>[3x]GLPRVAVDLVAPPLVHPHSQVAAGAPKVVQFRMSIEEKKMVADDDGTTAQAMTFNGSVPGPTLVVHEGDYIELTLVNPATNSMPHNVDFHAATGALGGAGLTQVVPGQEAVLRFKADRSGTFVYHCAPAGMVPWHVVSGMNGALMVLPRDGLRDAAGAALAYDRVYTIGESDLYVPKAADGNYSDYPAL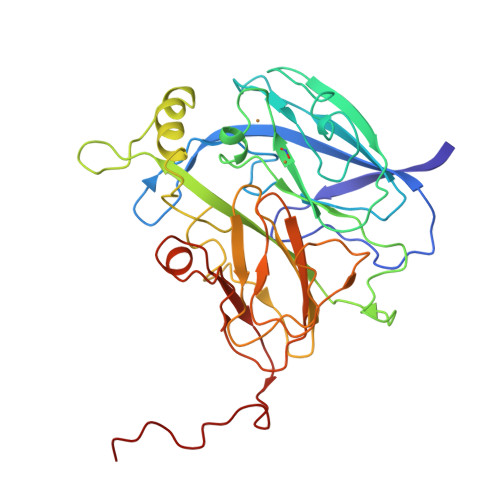ASAYADTVAVMRTLTPSHAVFNGAVGALTGANALTAAVGESVLIIHSQANRDSRPHLIGGHGDWVWTTGKFANPPQLNMETWFIPGGSAAAALYTFKQPGTYAYLSHNLIEAMELGAAAQASVEGQWDDDLMTSVAAPGPA> FTDVP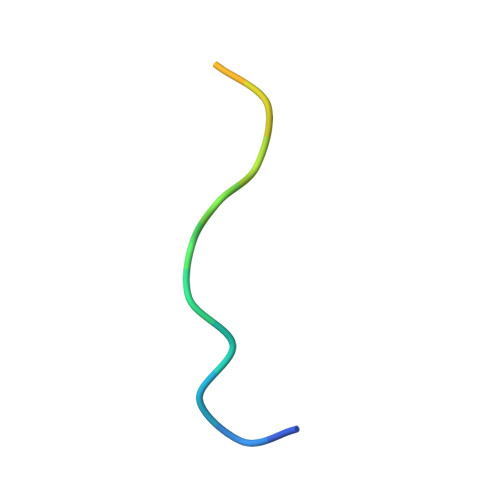ALNYPATPPPH> MKETAAAKFERQHMDSSTSAASSSNYCNQMMKSRNLTKDRCKPVNTFVHESLADVQAVCSQKNVACKNGQTNCYQSYSTMSITDCRETGSSKYPNCAYKTTQAN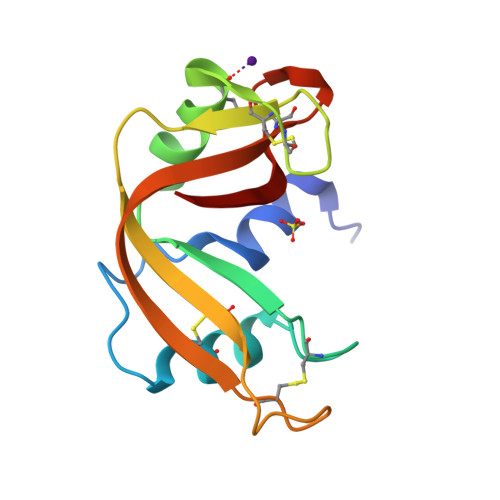KHIIVACEGNGYVPVHFDASV6-(4-methylphenyl)quinazoline-2,4-diamine | C15 H14 N4 | 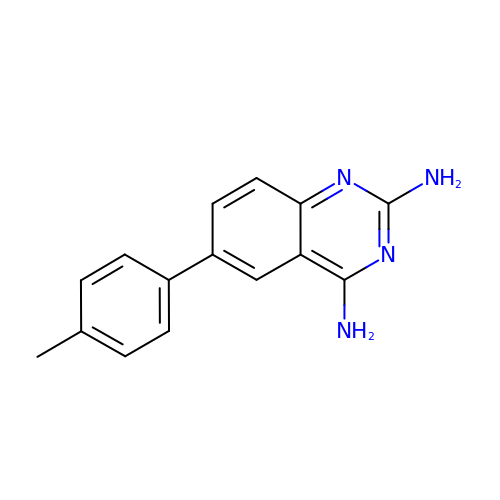NTHVHSAKVYNNGQ-UHFFFAOYSA-N> DVVVQAPTQVPGFLGDSVTLPCYLQVPNMEVTHVSQLTWARHGESGSMAVFHQTQGPSYSESKRLEFVAARLGAELRNASLRMFGLRVEDEGNYTCLFVTFPQGSRSVDIWLRVLAKPQNTAEVQKVQLTGEPVPMARCVSTGG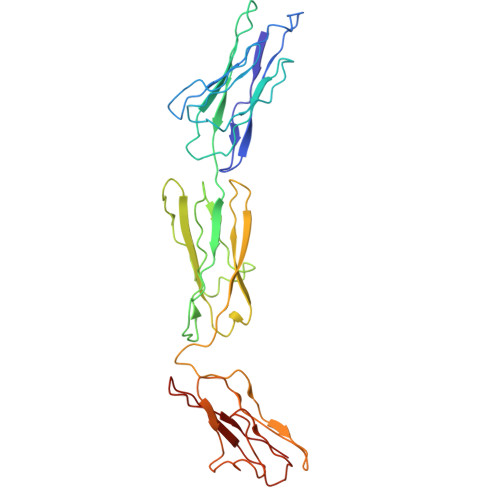RPPAQITWHSDLGGMPNTSQVPGFLSGTVTVTSLWILVPSSQVDGKNVTCKVEHESFEKPQLLTVNLTVYYPPEVSISGYDNNWYLGQNEATLTCDARSNPEPTGYNWSTTMGPLPPFAVAQGAQLLIRPVDKPINTTLICNVTNALGARQAELTVQV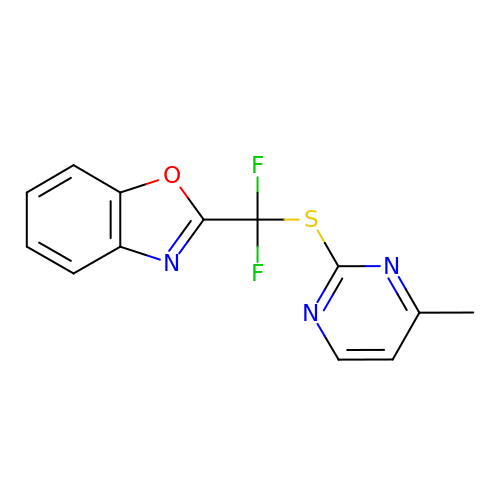2-[DIFLUORO-[(4-METHYL-PYRIMIDINYL)-THIO]METHYL]-BENZOXAZOLE | C13 H9 F2 N3 O S | VJAIXDQDRKEAAZ-UHFFFAOYSA-N> SLSNKLTLDKLDVKGKRVVM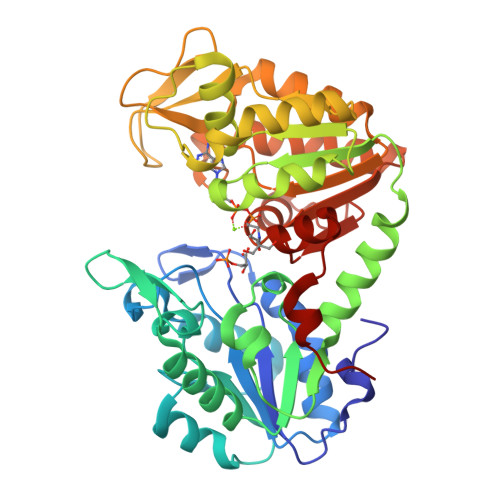RVDFNVPMKNNQITNNQRIKAAVPSIKFCLDNGAKSVVLMSHLGRPDGVPMPDKYSLEPVAVELKSLLGKDVLFLKDCVGPEVEKACANPAAGSVILLENLRFHVEEEGKGKDASGNKVKAEPAKIEAFRASLSKLGDVYVNDAFGTAHRAHSSMVGVNLPQKAGGFLIKKELNYFAKALESPERPFLAILGGAKVADKIQLINNMLDKVNEMIIGGGMAFTFLKVLNNMEIGTSLFDEEGAKIVKDLMSKAEKNGVKITLPVDFVTADKFDENAKTGQATVASGIPAGWMGLDCGPESSKKYAEAVTRAKQIVWNGPVGVFEWEAFARGTKALMDEVVKATSRGCITIIGGGDTATCCAKWNTEDKVSHVSTGGGASLELLEGKVLPGVDALSNI S-(N-HYDROXY-N-IODOPHENYLCARBAMOYL)GLUTATHIONE | C17 H23 I N4 O8 S | 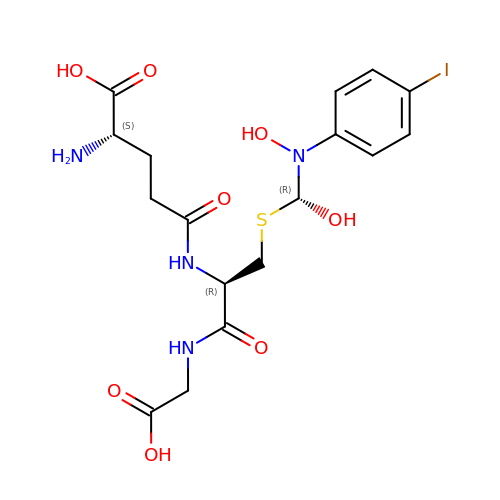SCHAHXXLASZJCD-NVGCLXPQSA-N>MYEFKDYYQNTVQLSFDDQPFSDSPKHVWVICRFGGKWLLTEHEDRGYEFPGGKVEPMECAEEAALREVKEETGARVKSLKYLGQYKVLGKEKVIVKNI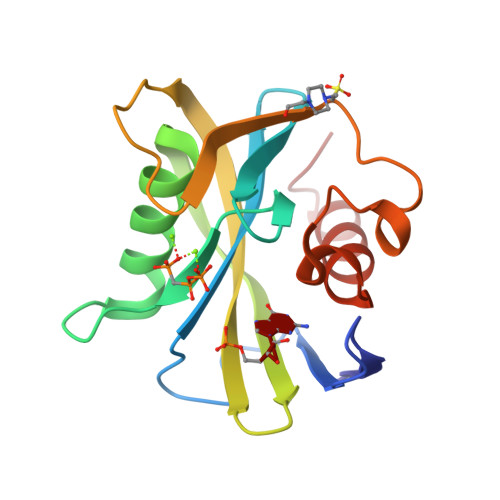YFADIEKLEKQADYFETKGPVLFHELPENLSRNKKFSFIMKDSVLPISLKKLKESGWIE[2x]(7R)-7-methyl-2-[(3-oxo-2,3-dihydro-1H-indazol-6-yl)amino]-5,8-di(prop-2-yn-1-yl)-7,8-dihydropteridin-6(5H)-one | C20 H17 N7 O2 | 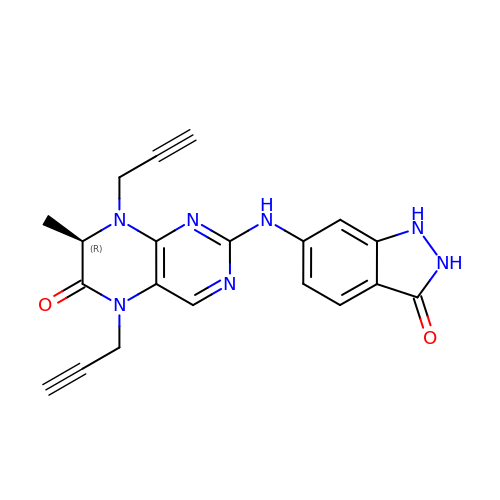GDTXGHSGLKEJJP-GFCCVEGCSA-N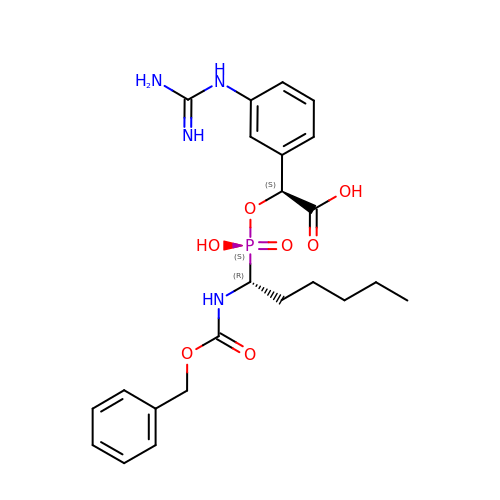(5R,6S,8S)-8-(3-{[AMINO(IMINO)METHYL]AMINO}PHENYL)-6-HYDROXY-3-OXO-5-PENTYL-1-PHENYL-2,7-DIOXA-4-AZA-6-PHOSPHANONAN-9-OIC ACID 6-OXIDE | C23 H31 N4 O7 P | XFGOBDZHGXXQBF-UXHICEINSA-N>[2x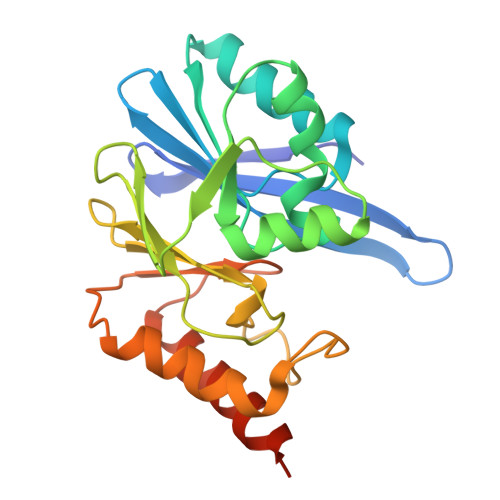]SQGHKPLEVIKIEDGVYLHTSFKNIEGYGLVDSNGLVVLDNNQAYIIDTPWSEEDTKLLLSWATDRGYQVMASISTHSHEDRTAGIKLLNSKSIPTYTSELTKKLLAREGKPVPTHYFKDDEFTLGNGLIELYYPGAGHTEDNIVAWLPKSKILFGGCLVRSHEWEGLGYVGDASISSWADSIKNIVSKKYPIQMVVPGHGKVGSSDILDHTIDLAESASNKLMQPTAEASAD> GEIEFIESSKDAGFPVINTPSKTKLEPSVFHQVFEGNKEPAVLRSGDPRLKANF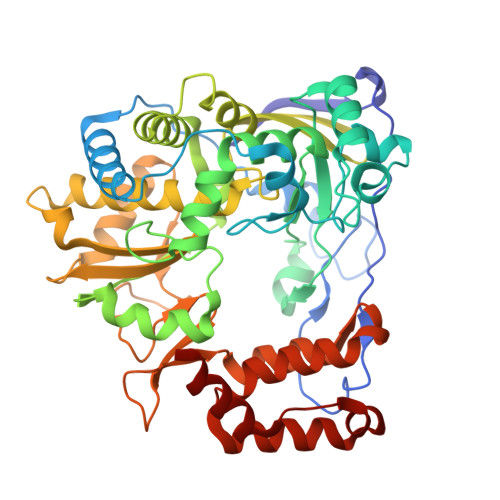EEAIFSKYIGNVNTHVDEYMLEAVDHYAGQLATLDISTEPMKLEDAVYGTEGLEALDLTTSAGYPYVALGIKKRDILSKKTKDLTKLKECMDKYGLNLPMVTYVKDELRSIEKVAKGKSRLIEASSLNDSVAMRQTFGNLYKTFHLNPGVVTGSAVGCDPDLFWSKIPVMLDGHLIAFDYSGYDASLSPVWFACLKMILEKLGYTHKETNYIDYLCNSHHLYRDKHYFVRGGMPSGCSGTSIFNSMINNIIIRTLMLKVYKGIDLDQFRMIAYGDDVIASYPWPIDASLLAEAGKGYGLIMTPADKGECFNEVTWTNVTFLKRYFRADEQYPFLVHPVMPMKDIHESIRWTKDPKNTQDHVRSLCLLAWHNGEHEYEEFIRKIRSVPVGRCLTLPAFSTLRRKWLDSF>MHHHHHHMRMIQKFEGKKPEIHETAFVHPRATIIGDVEIGPKTSVWPGAVIRADIEKITIGKNTCIKDNAVIHPADVYHEEEIEYVPVKIGDNNIIGHRALIHGAKINDESIVGAGSIVFNKAEVKTNSMVGMGAVVLEKQEVPNGKIVVGIPARVLRELEEREIKQIKKQADTHAELAEHYSREIEEP[5x]

CAs (E.C. 4.2.1.1) are ubiquitous metalloenzymes that catalyze the reversible hydration of carbon dioxide to bicarbonate (CO2 + H2O ⇋ HCO3– + H+). Here, we report on the first crystal structure of a halophilic γ-class CA (CA_D). The gene was derived from SAG analysis of an uncultured archaeon from the Red Sea Discovery Deep brine pool and was identified using the PPM algorithm. The gene was expressed in the bioengineered haloarchaeon Halobacterium sp. NRC-1.

The monomer contains a seven-turn, left-handed β-helix connected to an α-helix running antiparallel to the β-helix axis. For example, CA_D contains a connecting β-sheet, while Cam consists of an additional α-helix instead. Notably, CA_D is organized into trimers, resembling the reported active conformation for γ-CAs, where the active site includes residues from the adjacent monomers. Closer inspection of the active site reveals a zinc ion, coordinated by three histidine residues (His64 chain A, His89 chain B, and His94 chain A). A well-defined water molecule is coordinated to the zinc ion, which acts as the nucleophile in the reaction mechanism of these enzymes. Interestingly, one half of the active site pocket exhibits a more hydrophobic character whereas the facing side is more hydrophilic. The CA_D trimer displayed an increased number of hydrogen bonds and salt bridges compared to all of the individual meso- and thermophilic homologs being additionally added to the enzyme upon trimerization (hydrogen bonds: 69 vs. homolog average of 42; salt bridges: 10 vs. a homolog average of 5 or 5.5). The CA_D trimer contains an overall negative surface potential, while a positive charge is located only in two concentrated locations. The CA_D trimer protein surface contains a decreased number of hydrophobic and polar amino acid residues whilst showing an increased number of charged amino acid residues on the surface as compared to homologs. A closer look at positively and negatively charged amino acids on the trimer surface of CA_D reveals the dominance of glutamate (23.6 vs. 10.5 and 14.4% on the surface of mesophilic and thermophilic homologs, respectively).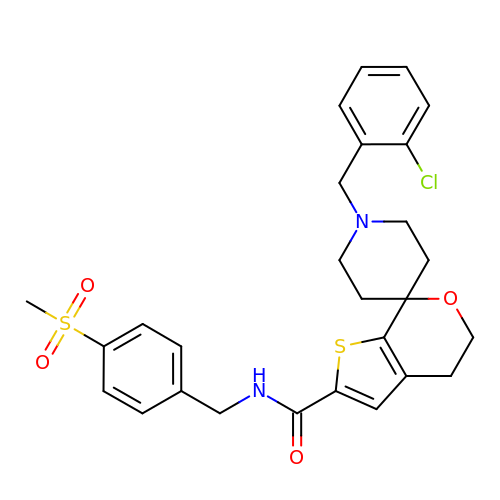1-[(2-chlorophenyl)methyl]-N-{[4-(methylsulfonyl)phenyl]methyl}-4',5'-dihydrospiro[piperidine-4,7'-thieno[2,3-c]pyran]-2'-carboxamide | C27 H29 Cl N2 O4 S2 | FADIARAUFGUAAD-UHFFFAOYSA-N> GSHMMEAILNKNMKILIVDDFSTMRRIVKNLLRDLGFNNTQEADDGLTALPMLKKGDFDFVVTDWNMPGMQGIDLLKNIRADEELKHLPVLMITAEAKREQIIEAAQAGVNGYIVKPFTAATLKEKLDKIFERL

Vibrio cholerae contains multiple copies of chemotaxis response regulator (VcCheY1–VcCheY4) whose functions are elusive yet. Autophosphorylated CheA then donates phosphate to the response regulator CheY. Phosphorylated CheY interacts with the flagellar motor protein FliM and influence the direction of flagellar rotation from counter clock wise (CCW) to clock wise (CW). As expected, both VcCheY3 and VcCheY4 possess (β/α)5 fold typical of the response regulators.

We have solved the structures of VcCheY3 in Ca2+ and Mg2+ bound states to the resolutions of 1.67 Å and 2.2 Å respectively. The Ca2+ (or Mg2+) of VcCheY3 is heptacoordinated where four coordinations occur with protein atoms and three with water molecules. The average coordination distance between Ca2+ and the protein atoms is about 2.4 Å while this is of about 2.1 Å in case of Mg2+ which is due to the size difference of the ions. D60 is the site of phosphorylation in VcCheY3 as it corresponds to D57 of StCheY. Both in the Mg2+ and Ca2+ bound free state structures of VcCheY3, the side chain of W61 (that corresponds to W58 of StCheY) is observed in a conformation, substantially different from that of StCheY. In the free state structure of VcCheY3, the side chain of W61 buries unusually deeply with a χ1 of −135° and χ2 of −133°. Y109 stays in its ‘out’ position and the side chain of M88 (with χ1 of 64°, χ2 of 175°) stays between W61 and Y109, packing snugly with W61, Y109 and V106 through hydrophobic interactions. This packing essentially fills up the pocket, required for the ‘inward’ positioning of Y109 upon activation. Moreover, in this inactivated structure of VcCheY3, the crucial T90 of β4α4 loop (that corresponds to T87 of StCheY), which stabilizes the bound phosphate on D60 upon activation, is hydrogen bonded with Q97. To the best of our knowledge, this kind of interaction involving the Thr of β4α4 loop was not observed so far in any other response regulator. In VcCheY3, T90 and Q97 are oriented in such a fashion that together they form a capping on the aforesaid hydrophobic packing and at the same time block the ‘out to in’ trajectory of Y109. Therefore, the hydrophobic packing of W61 with M88 and V106, together with the hydrogen bond between T90 and Q97 and the water mediated interaction between W61 and E100 seem to make a conformational barrier that may affect the process of activation in VcCheY3.5-O-phosphono-D-xylulose | C5 H11 O8 P 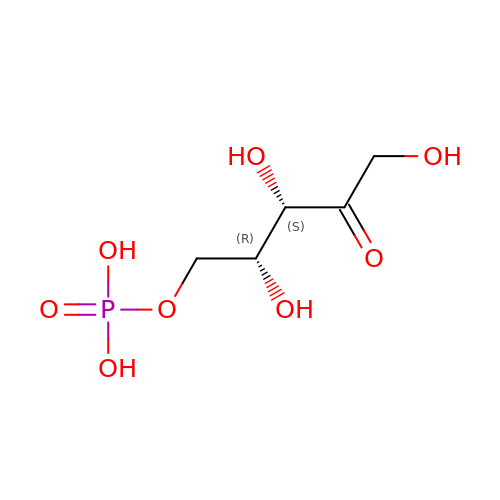| FNZLKVNUWIIPSJ-RFZPGFLSSA-N> MTVRKNQATLTADEKRRFVAAVLELKRSGRYDEFVRTHNEFIMSDTDSGERTGHRSPSFLPWHRRFLLDFEQALQSVDSSVTLPYWDWSADRTVRASLWAPDFLGGTGRSTDGRVMDGPFAASTGNWPINVRVDSRTYLRRSLGGSVAELPTRAEVESVLAISAYDLPPYNSASEGFRNHLEGWRGVNLHNRVHVWVGGQMATGVSPNDPVFWLHHAYVDKL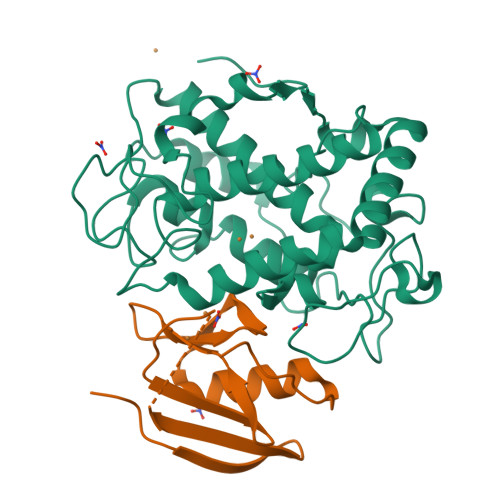WAEWQRRHPDSAYVPTGGTPDVVDLNETMKPWNTVRPADLLDHTAYYTFDALEHHHHHH;> MPEITRRRALTAAAAVAATASAAVTLAAPAASAAGHHEPAAPESFDEVYKGRRIQGRPAGGGAHHHEHGGGYEVFVDGVQLHVMRNADGSWISVVSHYDPVPTPRAAARAAVDELQGAPLLPFPANLEHHHHHH> APITAPDITSICKDASSGIGNQEGAIRTRKCCPPSLGKKIKDFQFPNDKKVRMRWPAHKGTKKQVDDYRR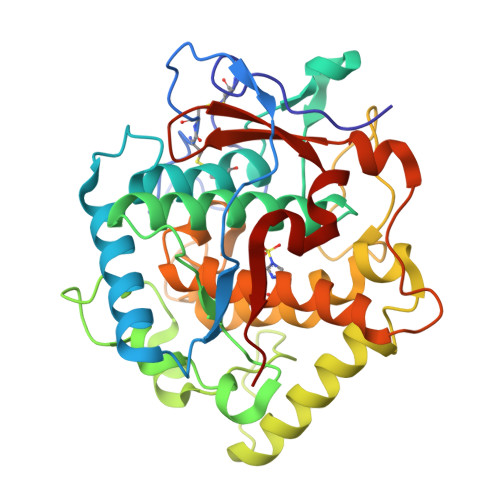AIAAMRALPDDDPRSFVSQAKIHCAYCNGGYTQVDSGFPDIDIQIHNSWLFFPFHRWYLYFYERILGSLIDEPNFALPYWKWDEPKGMPISNIFLGDASNPLYDQYRDANHIEDRIVDLDYDGKDKDIPDQQQVACNLSTVYRDLVRNGVDPTSFFGGKYVAGDSPVANGDPSVGSVEAGSHTAVHRWVGDPTQPNNEDMGNFYSAGYDPVFYIHHANVDRMWKLWKELRLPGHVDITDPDWLNASYVFYDENKDLVRVYNKDCVNLDKLKYNFIENSKE>[2x]MNDFHRDTWAEVDLDAIYDNVENLRRLLPDDTHIMAVVKANAYGHGDVQVARTALEAGASRLAVAFLDEALALREKGIEAPILVLGASRPADAALAAQQRIALTVFRSDWL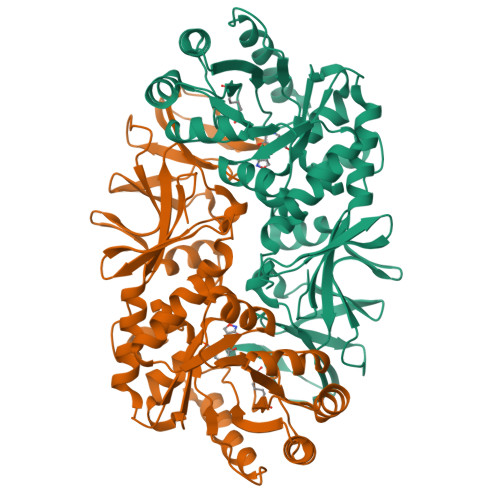EEASALYSGPFPIHFHLKMDTGMGRLGVKDEEETKRIVALIERHPHFVLEGLYTHFATADEVNTDYFSYQYTRFLHMLEWLPSRPPLVHCANSAASLRFPDRTFNMVRFGIAMYGLAPSPGIKPLLPYPLKEAFSLHSRLVHVKKLQPGEKVSFGATYTAQTEEWIGTIPIGYADGWLRRLQHFHVLVDGQKAPIVGRICMDQCMIRLPGPLPVGTKVTLIGRQGDEVISIDDVARHLETINYEVPCTISYRVPRIFFRHKRIMEVRNAIGRGESSA> GPP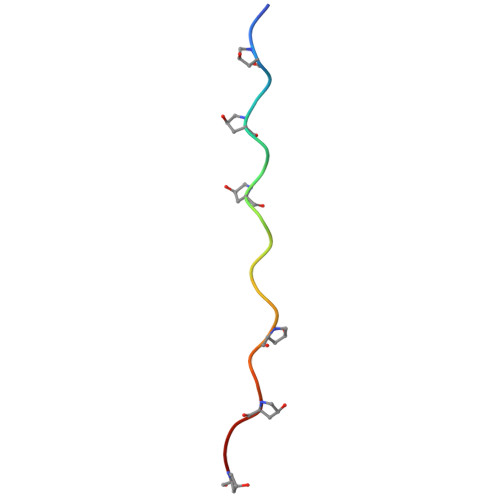GPPGPPGPAGFPGPPGPP>SLRSDLINALYDENQKYDVCGIISAEGKIYPLGSDTKVLSTIFELFSRPIINKIAEKHGYIVEEPKQQNHY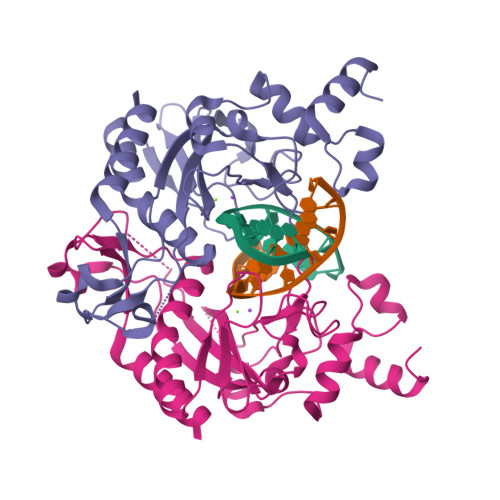PDFTLYKPSEPNKKIAIDIATTYTNKENEKIKFTLGGYTSFIRNNTKNIVYPFDQYIAHWIIGYVYTRVATRKSSLKTYNINELNEIPKPYKGVKVFLQDKWVIAGDLAGSGNTTNIGSIHAHYKDFVEGKGIFDSEDEFLDYWRNYERTSQLRNDKYNNISEYRNWIYRGRK[2x]Within this complex, UvrA acts as the initial damage sensor but hands off the lesion-containing DNA to UvrB and dissociates, leaving UvrB bound to the lesion in a preincision complex, the precise nature of which is not known. Both UvrA and UvrB expend ATP to form the preincision complex, which is believed to require threading of a β-hairpin element on UvrB through the DNA duplex. UvrB presents the lesion-containing strand to UvrC, which catalyzes hydrolysis of the 5th phosphodiester bond 3′ to the lesion and then the 8th phosphodiester bond 5′ to the lesion. UvrB is classified as a member of SF2 helicases on the basis of conserved helicase motifs (I-VI) (Supplementary ).

We therefore introduced a mutant Cys residue into the hydrophobic pocket and disulfide-crosslinked the resulting UvrB(T251C) protein to a single-stranded DNA substrate containing a thiol-tethered nucleobase, a cytosine. The complimentary strand is designed to contain two pyrimidine-pyrimidine mismatches on the immediate 5′ side of the modified cytosine; these were introduced to destabilize the duplex in the region expected to form a bubble, thereby facilitating maintenance of the helix-penetrated state for the β-hairpin. We determined crystal structures of UvrB disulfide-crosslinked to a 20-mer duplex substrate, in both the presence and absence of ATP, at 2.6 Å and 2.8 Å resolution, respectively. For those crystals grown in the presence of ATP, we clearly observe a nucleotide bound to the ATP binding site located at the interdomain cleft within helicase domain. However, the electron density corresponds to ADP plus inorganic phosphate; hence we conclude that the ATPase site retains activity in our crosslinked complex. As expected on the basis of the synthetic crystallography approach used to trap these structures, the 13th nucleobase on the inner strand, a cytosine, is extruded from the duplex and inserted into the hydrophobic pocket between domains 1a and 1b. As predicted, in our structures the β-hairpin loop was found to be fully inserted between the two DNA strands, clamping the inner strand between the β-hairpin and domain 1b (Figures 3a–3(c)). Though insertion of the β-hairpin loop requires disruption of only one or two base-pairs at the insertion site, our structures reveal disruption of base-pairing throughout the entire 6 bp duplex region comprising the crosslinked cytosine. The outer strand also makes contacts to UvrB, but these comprise almost exclusively van der Waals interactions. In agreement with previous EM studies, the UvrB-bound DNA contains a sharp bend (~60°) localized at the junction between the bubble and the fully base-paired segment flanking on its left side (“left flank,” Figure 3d). If so, the observed contacts between the helicase motifs engaged in DNA binding and the inner strand phosphates suggest that our structures obtained in both the presence and absence of ATP (hydrolyzed to ADP and Pi in crystallo) represent “open” states.

>[2x]VEGRFQLVAPYEPQGDQPQAIAKLVDGLRRGVKHQTLLGATGTGKTFTISNVIAQVNKPTLVIAHNKTLAGQLYSELKEFFPHNAVEYFVSYYDYYQPEAYVPQTDTYIEKDAKINDEIDKLRHSATSALFERRDVIIVASVSSIYGLGSPEEYRELVVSLRVGMEIERNALLRRLVDIQYDRNDIDFRRGTFRVRGDVVEIFPASRDEHSIRVEFFGDEIERIREVDALTGEVLGEREHVAIFPASHFVCREEKMRLAIQNIEQELEERLAELRAQGKLLEAQRLEQRTRYDLEMMREMGFSSGIENYSRHLALRPPGSTPYTLLDYFPDDFLIIVDESHVTLPQLRGMYNGDRARKQVLVDHGFRLPSALDNRPLTFEEFEQKINQIIYVSATPGPYELEHSPGVVEQIIRPTGLLDPTIDVRPTKGQIDDLIGEIRERVERNERTLVTTLTKKMAEDLTDYLKEAGIKVAYLHSEIKTLERIEIIRDLRLGKYDVLVGINLLREGLDIPEVSLVAILDADKEGFLRSERSLIQTIGRAARNANGHVIMYADTITKSMEIAIQETKRRRAIQEEYNRKHGIVPRTVKKEIR>[2x]GSGHWGAWMPSTISAFEGTCVSIPCRF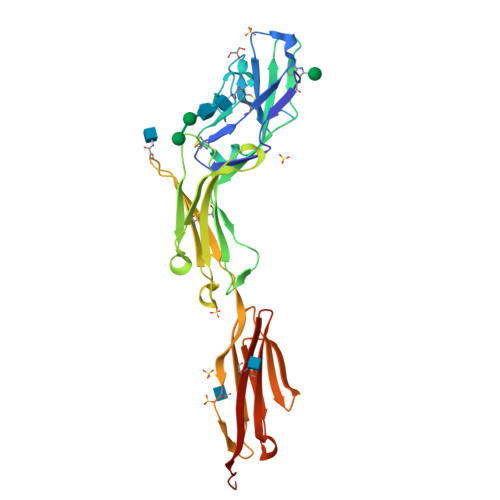DFPDELRPAVVHGVWYFNSPYPKNYPPVVFKSRTQVVHESFQGRSRLLGDLGLRNCTLLLSTLSPELGGKYYFRGDLGGYNQYTFSEHSVLDIVNTPNIVVPPEVVAGTEVEVSCMVPDNCPELRPELSWLGHEGLGEPTVLGRLREDEGTWVQVSLLHFVPTREANGHRLGCQAAFPNTTLQFEGYASLDVKYPPVIVEMNSSVEAIEGSHVSLLCGADSNPPPLLTWMRDGMVLREAVAKSLYLDLEEVTPGEDGVYACLAENAYGQDNRTVELSVMYAAAAHHHHHH3-propyl-2-oxoglutarate | C8 H12 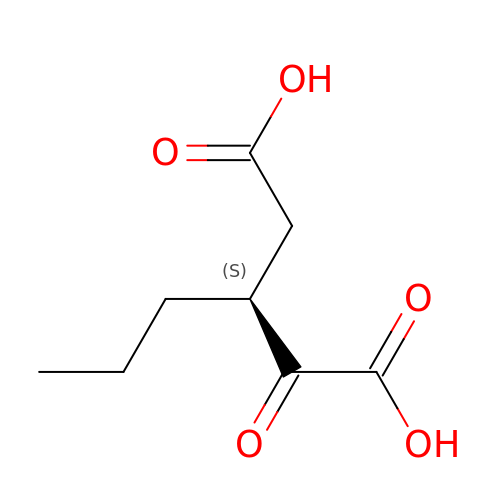O5 | RICKOBMVUQRAMO-YFKPBYRVSA-N>GRKERERLEEKLEDANERIAELVKLEERQRIARDLEDTLGQKLSLIGLKSDLARKLIYKDPEQAARELKSVQQTARTSLNEVRKIVSSMKGIRLKDELINIKQILEAADIMFIYEEEKWPENISLLNENILSMCLKEAVTNV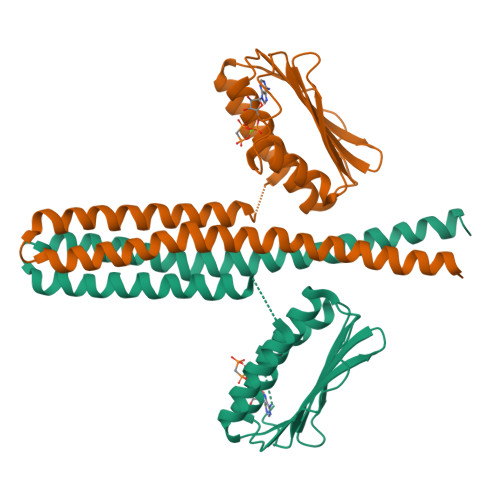VKHSQAKTCRVDIQQLWKEVVITVSDDGTFKGEENSFSKGHGLLGMRERLEFANGSLHIDTENGTKLTMAIPNNSK[2x]>MAHHHHHHMSQTVTTTIEYQVKDMSLASLGRKRIEMAEKEMPGLMACRAKYGEEKPLNGVRITGSLHMTVETAVLIETLKAIGGNIRWCSCNIFSTQDDAAAAIAAANTPVFAWKGETLVEYWECTWKAIRFGPYQGPQLIVDDGGDATLLIHRGFQAEKEPSILDEDGGVEELRIVNNLLKRILKEEPGFFSKIVPDIKGVSEETTTGVHRLYAMQKQGTLLFPAINVNDSVTKSKFDNIYGCRHSLLDGLNRATDVMLAGKECVICGFGDVGKGCAEALKGQGARVIVTEIDPINALQACMAGYTVKTVEDCLATADIYVTATGNKDIITLDHMKKMKDMAIICNIGHFDNEIDVLGLKTCEGVKEINIKPQVDQFLFPDGHSIILLAQGRLVNLGCATGHPAFVMSASFTNQTLAQISLWKDKYEIGVYTLP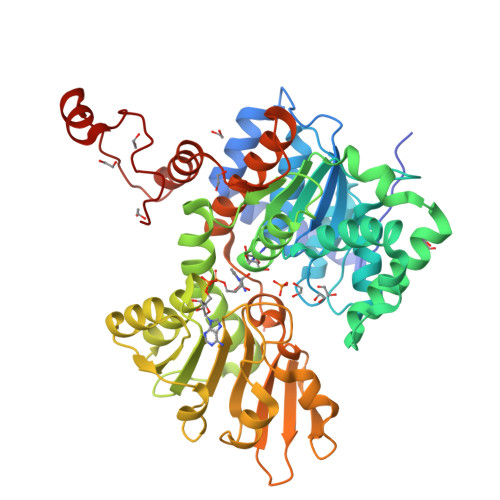KVLDEEVARLHLEKLGAKLTKLTTSQADYIGVNANGPYKADHYRY[4x]> MHHHHHHHHHHSGDEVDAGSGHMMCLECASAAAGGAEEEEADAERRRRRRGAQRGAGGSGCCGARGAGGAGVSAAGDEVQTLSGSVRRAPTGPPGTPGTPGCAATAKGPGAQQPKPASLGRGRGAAAAILSLGNVLNYLDRYTVAGVLLDIQQHFGVKDRGAGLLQSVFICSFMVAAPIFGYLGDRFNRKVILSCGIFFWSAVTFSSSFIPQQYFWLLVLSRGLVGIGEASYSTIAPTIIGDLFTKNTRTLMLSVFYFAIPLGSGLGYITGSSVKQAAGDWHWALRVSPVLGMITGTLILILVPATKRGHADQLGDQLKARTSWLRDMKALIRNRSYVFSSLATSAVSFATGALGMWIPLYLHRAQVVQKTAETCNSPPCGAKDSLIFGAITCFTGFLGVVTGAGATRWCRLKTQRADPLVCAVGMLGSAIFICLIFVAAKSSIVGAYICIFVGETLLFSNWAITADILMYVVIPTRRATAVALQSFTSHLLGDAGSPYLIGFISDLIRQSTKDSPLWEFLSLGYALMLCPF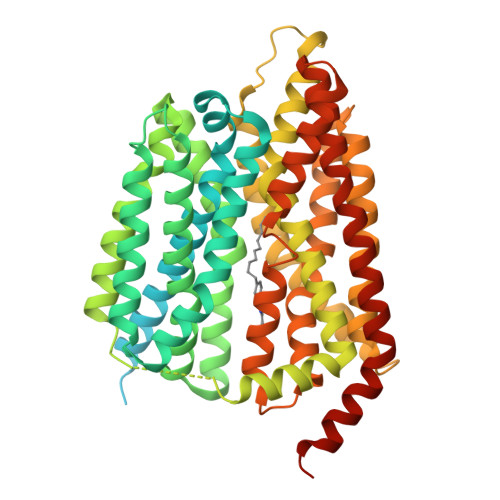VVVLGGMFFLATALFFVSDRARAEQQVNQLAMPPASVKV>[4x]MGITLGEVFPNFEADSTIGKLKFHD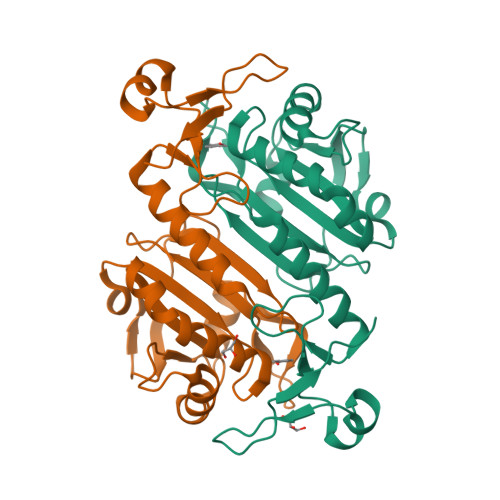WLGNSWGVLFSHPRDFTPVSTTELGRVIQLEGDFKKRGVKLIALSCDNVADHKEWSEDVKCLSGVKGDMPYPIIADETRELAVKLGMVDPDERTSTGMPLTCRAVFIIGPDKKLKLSILYPATTGRNFSEILRVIDSLQLTAQKKVATPADWQPGDRCMVVPGVSAEEAKTLFPNMEVKAVPSGKGYLRYTPQPKSMGGSRSHHHHHH1-(8-pyridin-2-ylpyrrolo[1,2-a]pyrimidin-6-yl)ethanone | C14 H11 N3 O | 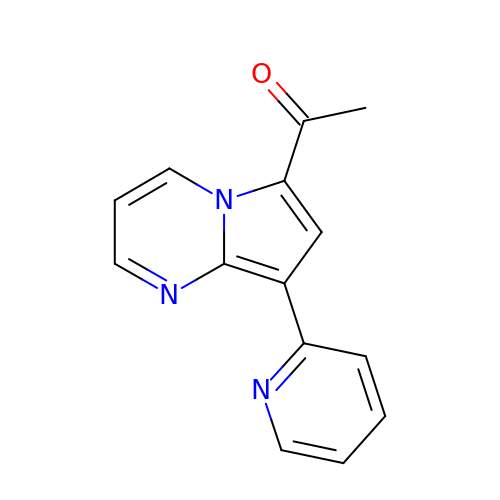LNUJODOPWTZPCA-UHFFFAOYSA-N5-(4-azanyl-1-propan-2-yl-pyrazolo[3,4-d]pyrimidin-3-yl)-1,3-benzoxazol-2-amine | C15 H15 N7 O | 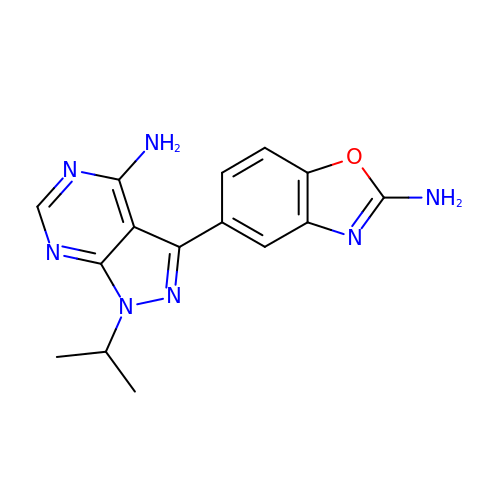GYLDXIAOMVERTK-UHFFFAOYSA-N2-chloro-1H-imidazole | C3 H3 Cl N2 | 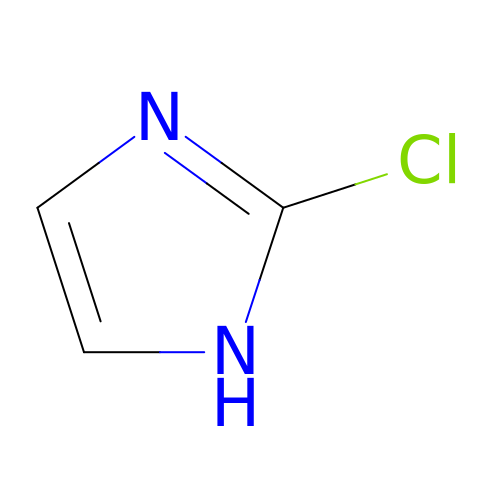OCVXSFKKWXMYPF-UHFFFAOYSA-N>GIDPFTM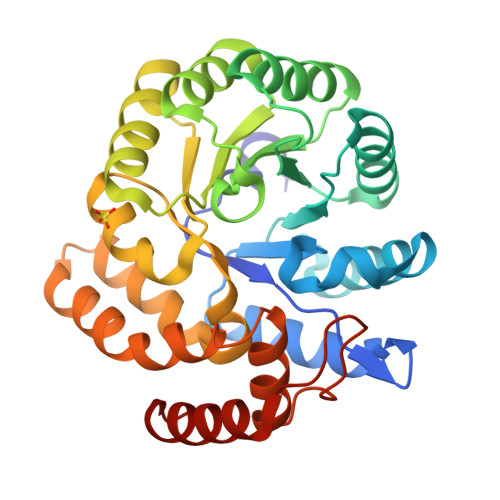FRGVGTAIVTPFKNGELDLESYERLVRYQLENGVNALIVLGTTGESPTVNEDEREKLVSRTLEIVDGKIPVIVGAGTNSTEKTLKLVKQAEKLGANGVLVVTPYYNKPTQEGLYQHYKYISERTDLGIVVYNVPGRTGVNVLPETAARIAADLKNVVGIKEANPAAAQIDRTVSLTKQARSDFMVWSGNDDRTFYLLCAGGDGVISVVSNVAPKQMVELCAEYFSGNLEKSREVHRKLRPLMKALFVETNPIPVKAALNLMGFIENELRLPLVPASEKTVELLRNVLKESGLL[4x]>[2x]MAPPVSERGLKSVVWRKIKTAVFDDCRKEGEWKIMLLDEFTTKLLSSCCKMTDLLEEGITVIENIYKNREPVRQMKALYFISPTPKSVDCFLRDFGSKSEKKYKAAYIYFTDFCPDSLFNKIKASCSKSIRRCKEINISFIPQESQVYTLDVPDAFYYCYSPDPSNASRKEVVMEAMAEQIVTVCATLDENPGVRYKSKPLDNASKLAQLVEKKLEDYYKIDEKGLIKGKTQSQLLIIDRGFDPVSTVLHELTFQAMAYDLLPIENDTYKYKTDGKEKEAVLEEDDDLWVRVRHRHIAVVLEEIPKLMKEISSTKKATEGKTSLSALTQLMKKMPHFRKQISKQVVHLNLAEDCMNKFKLNIEKLCKTEQDLALGTDAEGQRVKDSMLVLLPVLLNKNHDNCDKIRAVLLYIFGINGTTEENLDRLIHNVKIEDDSDMIRNWSHLGVPIVPPSQ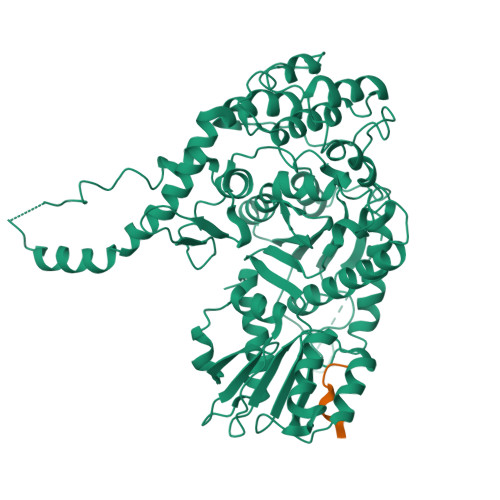QAKPLRKDRSAEETFQLSRWTPFIKDIMEDAIDNRLDSKEWPYCSRCPAVWNGSGAVSARQKPRTNYLELDRKNGSRLIIFVIGGITYSEMRCAYEVSQAHKSCEVIIGSTHILTPRKLLDDIKMLNKSKDKVSFKDE;>[2x]MRDRTHELRQ> GGDPHMMFGKKKNNGGSSTARYSAGNKYNTLSNNYALSAQQLLNASKIDDIDSMMGFERYVPPQYNGRFDAKDIDQIPGRVGWLTNMHATLVSQETLSSGSNGGGNSNDGERVTTNQGISGVDFYFLDEEGGSFKSTVVYDPYFFIACNDESRVNDVEELVKKYLESCLKSLQIIRKEDLTMDNHLLGLQKTLIKLSFVNSNQLFEARKLLRPILQDNANNNVQRNIYNVAANGSEKVDAKHLIEDIREYDVPYHVRVSIDKDIRVGKWYKVTQQGFIEDTRKIAFAD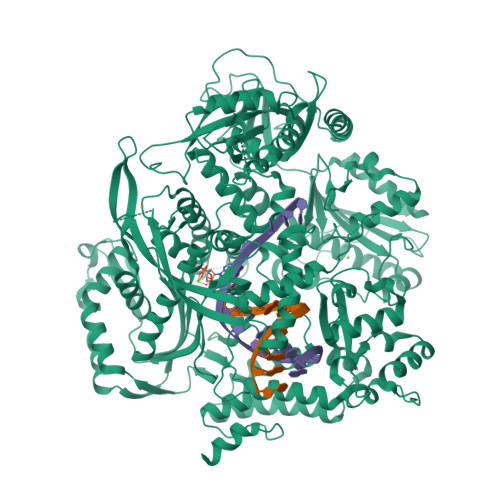PVVMAFDIETTKPPLKFRDSAVDQIMMISYMIDGEGFLITNREIISEDIEDFEYTPKPEYPGFFTIFNENDEVALLQRFFEHIRDVRPTVISTFNGDFFDWPFIHNRSKIHGLDMFDEIGFAPDAEGEYKSSYCSHMDCFRWVKRDSYLPQGSQGLKAVTQSKLGYNPIELDPELMTPYAFEKPQHLSEYSVSDAVATYYLYMKYVHPFIFSLCTIIPLNPDETLRKGTGTLCEMLLMVQAYQHNILLPNKHTDPIERFYDGHLLESETYVGGHVESLEAGVFRSDLKNEFKIDPSAIDELLQELPEALKFSVEVENKSSVDKVTNFEEIKNQITQKLLELKENNIRNELPLIYHVDVASMYPNIMTTNRLQPDSIKAERDCASCDFNRPGKTCARKLKWAWRGEFFPSKMDEYNMIKRALQNETFPNKNKFSKKKVLTFDELSYADQVIHIKKRLTEYSRKVYHRVKVSEIVEREAIVCQRENPFYVDTVKSFRDRRYEFKGLAKTWKGNLSKIDPSDKHARDEAKKMIVLYDSLQLAHKVILNSFYGYVMRKGSRWYSMEMAGITCLTGATIIQMARALVERVGRPLELDTDGIWCILPKSFPETYFFTLENGKKLYLSYPCSMLNYRVHQKFTNHQYQELKDPLNYIYETHSENTIFFEVDGPYKAMILPSSKEEGKGIKKRYAVFNEDGSLAELKGFELKRRGELQLIKNFQSDIFKVFLEGDTLEGCYSAVASVCNRWLDVLDSHGLMLEDEDLVSLICENRSMSKTLKEYEGQKSTSITTARRLGDFLGEDMVKDKGLQCKYIISSKPFNAPVTERAIPVAIFSADIPIKRSFLRRWTLDPSLEDLDIRTIIDWGYYRERLGSAIQKIITIPAALQGVSNPVPRVEHPDWLKRKIAT>GPGSSLSRFRGCLAGALLGDCVGSFYAAHDTVDLTSVLRHVQSLEPDPGTPGSERTEALYYTDDTAMARALVQSLLAKEAFDEVDMAHRFAQEYKKDPDRGYGAGVVTVFKKLLNPKCRDVFEPARAQFNGKGSYGNGGAMRVAGISLAYSSVQDVQKFARLSAQLTHASSLGYNGAILQALAVHLALQGESSSEHFLKQLLGHMEDLEGDAQSVLDARELGMEERPYSSRLKKIGELLDQASVTREEVVSELGNGIAAFESVPTAIYCFLRCMEPDPEIPSAFNSLQRTLIYSISLGG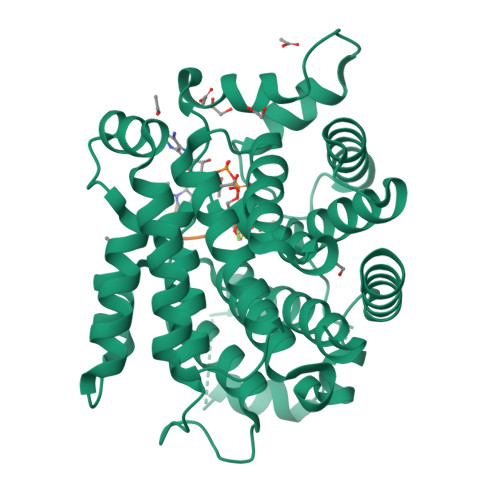DTDTIATMAGAIAGAYYGMDQVPESWQQSCEGYEETDILAQSLHRVFQKS[4x];>PAKSAPAPKKG[4x]>MTIVQAAQSRYSTK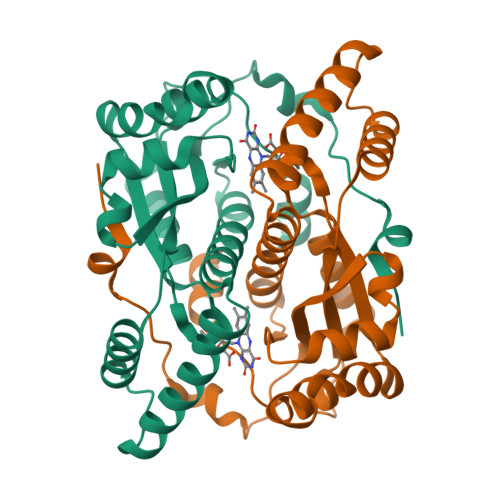AFDASRKLPEEKVAAVKELIRMSASSVNSQPWHFIVASSEEGKARIAKATQGGFAANERKILDASHVVVFCAKTAIDEAYLLDLLESEDKDGRYADVEAKNGMHAGRSFFVNMHRFDLKDAHHWMEKQVYLNVGTLLLGASAMEIDAVPIEGFDAKVLDEEFGLREKGFTSVVIVPLGYHSEDDFNAKLPKSRWSAETVFTEI[2x]methyl 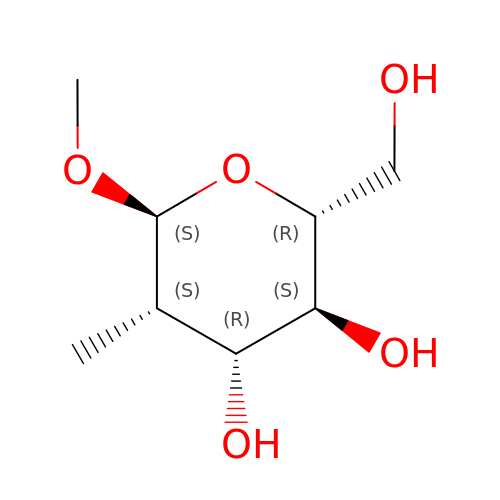2-deoxy-2-methyl-alpha-D-mannopyranoside | C8 H16 O5 | GNHGGSMJGHLAKR-WCMLQCRESA-N> NIGSQWRDDEVHFNRTLDSILVPRVVGSRGHQQVREYLVQSLNGLGFQTEVDEFKQRVPVFGELTFANVVGTINPQAQNFLALACHYDSKYFPNDPGFVGATDSAVPCAILLNTAKTLGAYLQKEFRNRSDVGLMLIFFDGEEAFK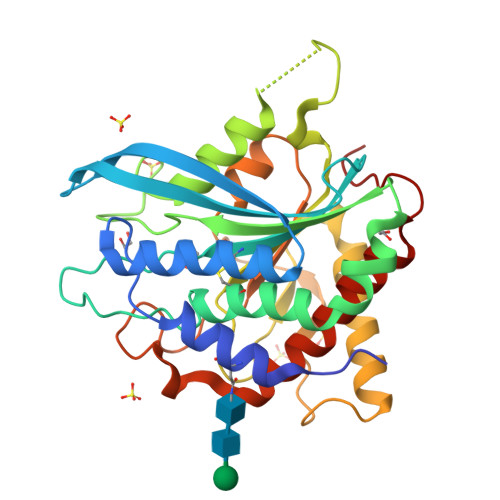EWTDADSVYGSKHLAAKLASKRSGSQAQLAPRNIDRIEVLVLLDLIGARNPKFSSFYENTDGLHSSLVQIEKSLRTAGQLEGNNNMFLSRVSGGLVDDDHRPFLDENVPVLHLVATPFPDVWHTPRDNAANLHWPSIRNFNRVFRNFVYQYLKRHTSPVNLRFYRT>[2x]MGQSKKLNKQPSSLSPLVQLAGIRKCFDGKEVIPQLDLTINNGEFLTLLGPSGCGKTTVLRLIAGLETVDSGRIMLDNEDITHVPAENRYVNTVFQSYALFPHMTVFENVAFGLRMQKTPAAEITPRVMEALRMVQLETFAQRKPHQLSGGQQQRVAIARAVVNKPRLLLLDQSLSALDYKLRKQMQNELKALQRKLGITFVFVTHDQEEALTMSDRIVVMRDGRIEQDGTPREIYEEPKNLFVAGFIGEINMFNATVIERLDEQRVRANVEGRECNIYVNFAVEPGQKLHVLLRPEDLRVEEINDDNHAEGLIGYVRERNYKGMTLESVV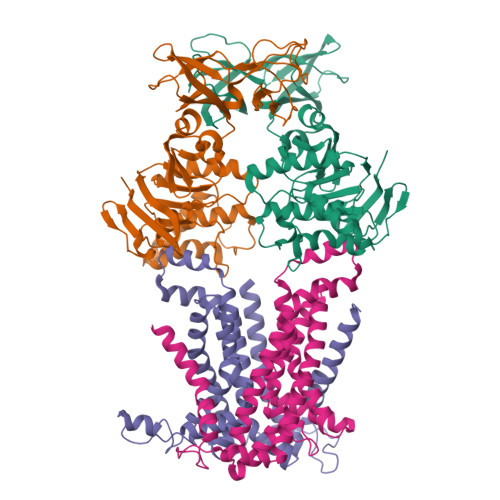ELENGKMVMVSEFFNEDDPDFDHSLDQKMAINWVESWEVVLADEEHK;> MKNTSKFQNVVIVTIVGWLVLFVFLPNLMIIGTSFLTRDDASFVKMVFTLDNYTRLLDPLYFEVLLHSLNMALIATLACLVLGYPFAWFLAKLPHKVRPLLLFLLIVPFWTNSLIRIYGLKIFLSTKGYLNEFLLWLGVIDTPIRIMFTPSAVIIGLVYILLPFMVMPLYSSIEKLDKPLLEAARDLGASKLQTFIRIIIPLTMPGIIAGCLLVMLPAMGLFYVSDLMGGAKNLLIGNVIKVQFLNIRDWPFGAATSITLTIVMGLMLLVYWRASRLLNKKVELE;> MIGRLLRGGFMTAIYAYLYIPIIILIVNSFNSSRFGINWQGFTTKWYSLLMNNDSLLQAAQHSLTMAVFSATFATLIGSLTAVALYRYRFRGKPFVSGMLFVVMMSPDIVMAISLLVLFMLLGIQLGFWSLLFSHITFCLPFVVVTVYSRLKGFDVRMLEAAKDLGASEFTILRKIILPLAMPAVAAGWVLSFTLSMDDVVVSSFVTGPSYEILPLKIYSMVKVGVSPEVNALATILLVLSLVMVIASQLIARDKTKGNTGDVK> MKISIYGAGNQRLYLEQLKVPEKFGGEPPYGGAGMAIEFAKAGHDVVL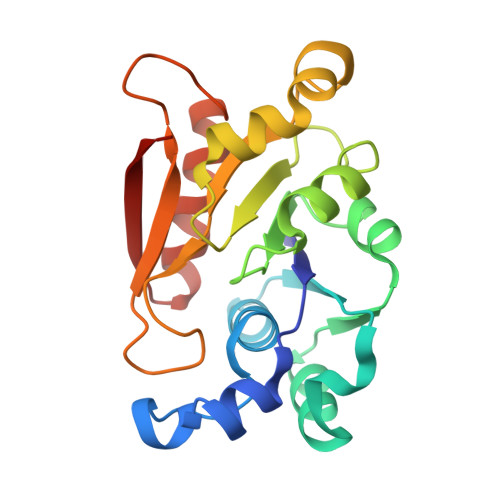SEPNRDVMSDDLWKKVEDAGVKVVSDDIEAAKHGEIHVLFTPFGRITLNIANTIIEHVPENAIICNTCTIPTPVLYRSLEGILRLKRRDVGISSMHPTGVPGTPSQKYYTIAGKALEGKEYATEDQINKLVELVKSVGKIPYVTPA> RSVYELDCIPLWGVVSIQGNRSEMEDAFAVSPHFLKLPIKMLMGDHEGMSPSATHLTGHFFGVYDGHGGHKVADYCRDRLHFALAEEIERIKDELCKRNTGEGRQVQWDKVFTSCFLTVDGEIEGKIGRAVVGSSDKVLEAVASETVGSTAVVALVCSSHIVVSNCGDSRAVLFRGKEAMPLSVDHKPDREDEYAR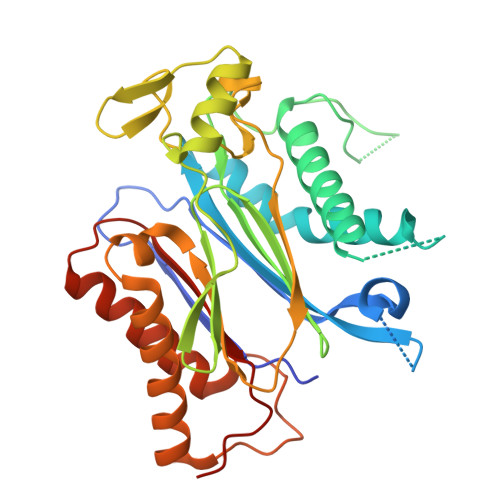IENAGGKVIQWQGARVFGVLAMSRSIGDRYLKPYVIPEPEVTFMPRSREDECLILASDGLWDVMNNQEVCEIARRRILMWHKKNGAPPLAERGKGIDPACQAAADYLSMLALQKGSKDNISIIVIDLKAQRKFKTRT> GSHMAGAQDFVPHTADLAELAAAAGECR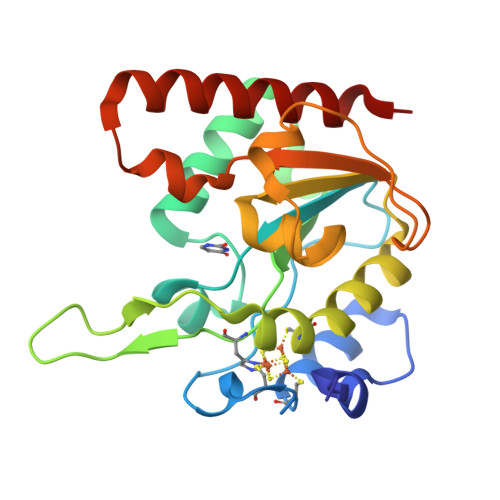GCGLYRDATQAVFGAGGRSARIMMIGEQPGDKEDLAGLPFVGPAGRLLDRALEAADIDRDALYVTNAVKHFKFTRAAGGKRRIAKTPSRTEVVACRPWLIAEMTSVEPDVVVLLGATAAKALLGNDFRVTQHRGEVLHVDDVPGDPALVATVHPSSLLRGPKEERESAFAGLVDDLRVAADVRP4-(4-{[4-(4-chlorophenyl)-5,6-dihydro-2H-pyran-3-yl]methyl}piperazin-1-yl)-N-{[3-nitro-4-(tetrahydro-2H-pyran-4-ylamino)phenyl]sulfonyl}benzamide 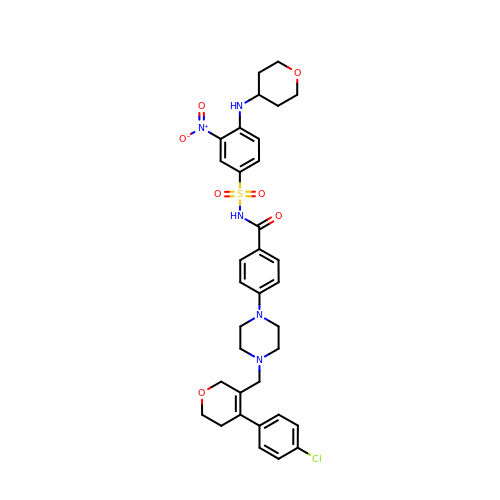| C34 H38 Cl N5 O7 S | AJWKZOOIFOHKSK-UHFFFAOYSA-N>[2x]EELPQIEIVQ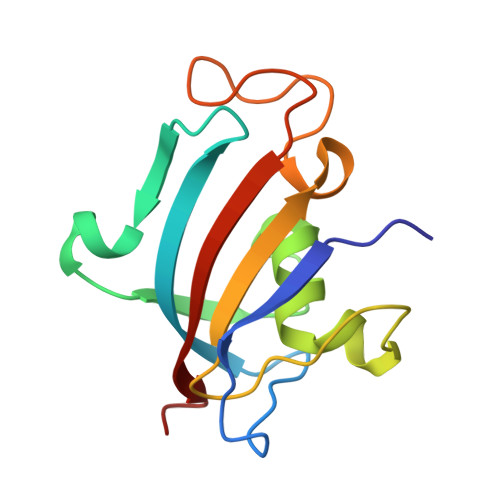EGDNTTFAKPGDTVTIHYDGKLTNGKEFDSSRKRGKPFTCTVGVGQVIKGWDISLTNNYGKGGANLPKISKGTKAILTIPPNLAYGPRGIPPIIGPNETLVFEVELLGVNGQ>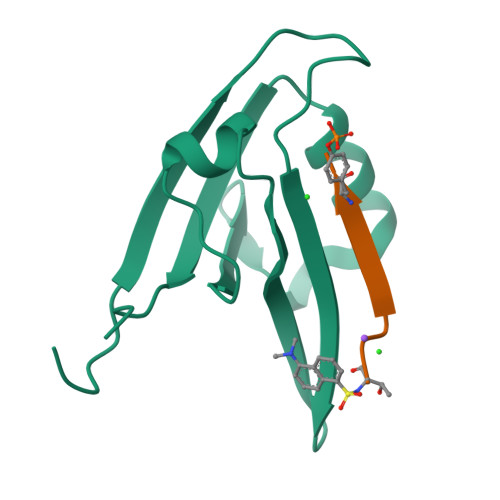 GAMGKVTHSIHIEKSDTAADTYGFSLSSVEEDGIRRLYVNSVKETGLASKKGLKAGDEILEINNRAADALNSSMLKDFLSQPSLGLLVRTYPEL;> TKQEEFYA>[2x]MAETVESSLA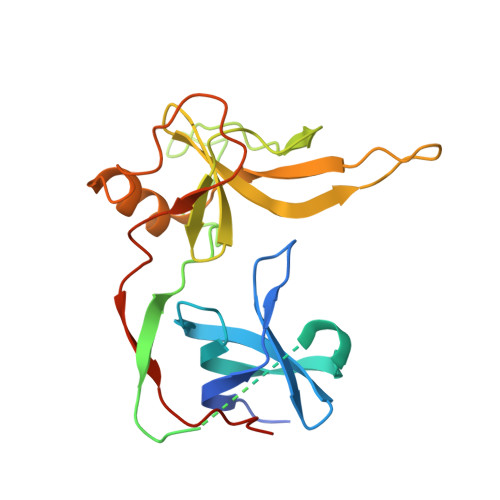KSHIEGSFTNVWKDDKTLDWYANYEGILWKATGVVVITGDETQVYAIWVPVGLAIPENEGGGSEGGGSEGGGSEGGGTKPPEYGDTPIPGYIYINPLDGTYPPGTEQNPANPNPSLEESHPLNTFMFQGNRFRNRQGALTVYTGTVTQGTDPVKTYYQYTPVSSKAMYDAYWNGKFRDVAFHSGFNEDPLVAEYQGQLSYLPQPPVNAPSGHHHHHH> KEALEIEKNSRKPPPYKHIKANKVIGKVQI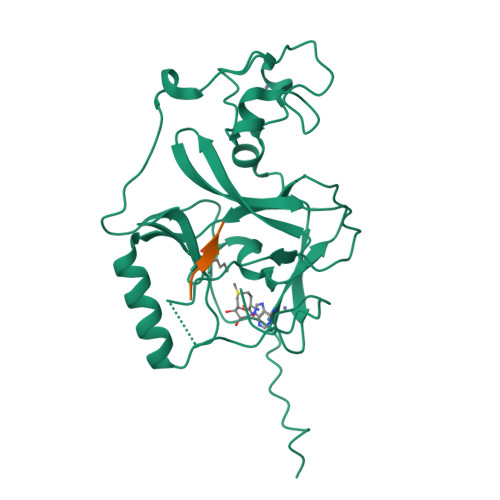QVADLSEIPRCNCKPADENPCGLESECLNRMLQYECHPQVCPAGDRCQNQCFTKRLYPDAEIIKTERRGWGLRTKRSIKKGEFVNEYVGELIDEEECRLRIKRAHENSVTNFYMLTVTKDRIIDAGPKGNYSRFMNHSCNPNCETQKWTVNGDVRVGLFALCDIPAGMELTFNYNLDCLGNGRTECHCGADNCSGFLG(3S)-6-(3-tert-butyl-5-{[(2,3-dichlorophenyl)carbamoyl]amino}-1H-pyrazol-1-yl)-1,2,3,4-tetrahydroisoquinoline-3-carboxylic 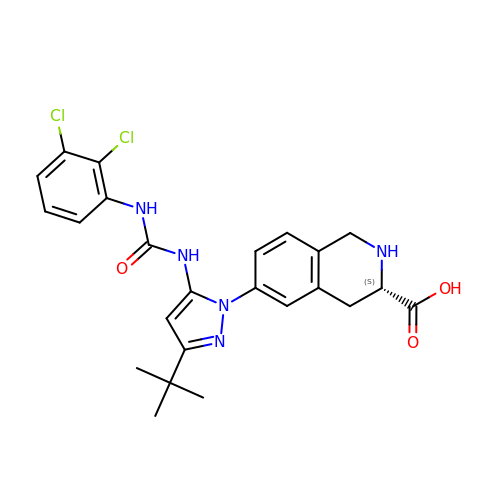acid | C24 H25 Cl2 N5 O3 | CMUVVEBHULJOFP-SFHVURJKSA-N>[2x]MPTVLASRVESDTTINVMKWKTVSTIFLVVVLYLIIGATV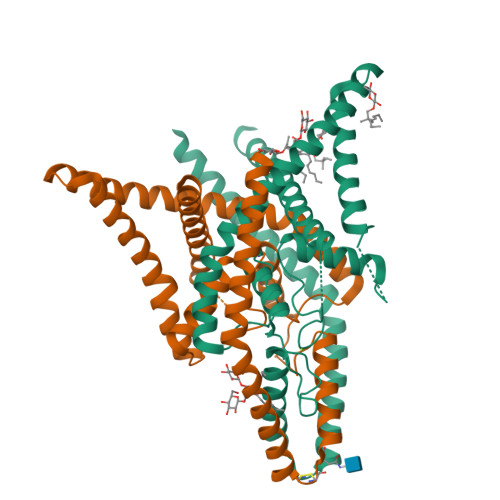FKALEQPHEISQRTTIVIQKQTFISQHSCVNSTELDELIQQIVAAINAGIIPLGNTSNQISHWDLGSSFFFAGTVITTIGFGNISPRTEGGKIFCIIYALLGIPLFGFLLAGVGDQLGTIFGKGIAKVEDTFIKWNVSQTKIRIISTIIFILFGCVLFVALPAIIFKHIEGWSALDAIYFVVITLTTIGFGDYVAGGSDIEYLDFYKPVVWFWILVGLAYFAAVLSMIGDWLRVISAENLYFQ>MRLAYVKNHEIYGEKLLGLTLRERIEKTLQRAGFDVRFFDELSLEEAEDYL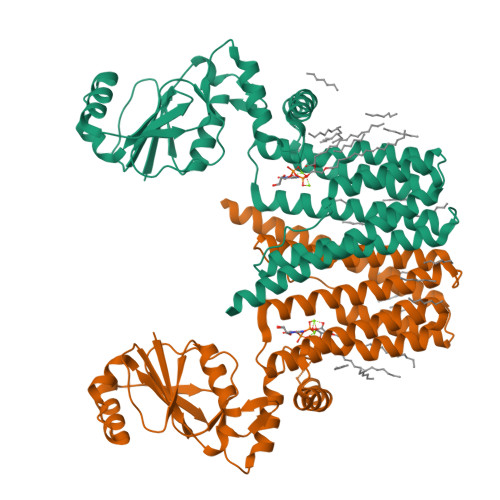IILEPVLILERDLLLEGRKILVSDGFTVGYFFGGDFRTVFDGNLQSSIEKYLSLNNLESYEIWAIKLSNDNLKTAEKLLLSSLIGSGSLNKYARGLFAAIFLPIARLLADWGVSPDAVTVVGTLGVMAGALIFYPMGQLFWGTVVITVFVFSDIIDGLMARLLFREGPWGAFLDSYLDRVGDSSVFTGIVIWFFLGGANPTIAILALICLVLSSLVSYSKARAEGLGLTANVGIAERSERLVVVLVATGLVGLGIPSWVLLVVLIVLAIASVVTIFQRVLTVREQAKAWTA[4x]> MRGSHHHHHHGSMTQVAKKILVTCASPYANGSIHLGHMLEHIQADVWVRYQRMRGHEVNFICADDAHGTPIMLKAQQLGITP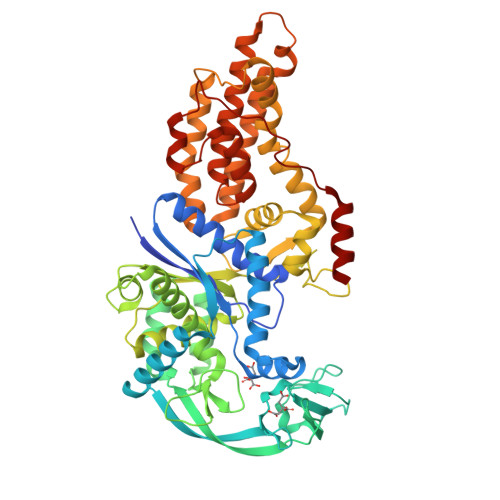EQMIGEMSQEHQTDFAGFNISYDNYHSTHSEENRQLSELIYSRLKENGFIKNRTISQLYDPEKGMFLPDRFVKGTCPKCKSPDQYGDNCEVCGATYSPTELIEPKSVVSGATPVMRDSEHFFFDLPSFSEMLQAWTRSGALQEQVANKMQEWFESGLQQWDISRDAPYFGFEIPNAPGKYFYVWLDAPIGLMGSFKNLCDKRGDSVSFDEYWKKDSTAELYHFIGKDIVYFLSLFWPAMLEGSNFRKPSNLFVHGYVTVNGAKMSKSRGTFIKASTWLNHFDADSLRYYYTAKLSSRIDDIDLNLEDFVQRVNADIVNKVVNLASRNAGFINKRFDGVLASELADPQLYKTFTDAAEVIGEAWESREFGKAVREIMALADLANRYVDEQAPWVVAKQEGRDADLQAICSMGINLFRVLMTYLKPVLPKLTERAEAFLNTELTWDGIQQPLLGHKVNPFKALYNRIDMRQVEALVEASK Legionella pneumophila is an opportunistic pathogen that causes the potentially fatal pneumonia known as Legionnaires’ disease. The pathology associated with infection depends on bacterial delivery of effector proteins into the host via the membrane spanning Dot/Icm type IV secretion system (T4SS). The Dot/Icm complex of L. pneumophila is one of the largest known T4SSs. The Dot/Icm T4SS has as many as 300 protein substrates, a striking contrast to the H. pylori Cag and B. pertussis Ptl T4SSs, each of which transports only one virulence factor.

Using 3D variability analysis, we reconstructed a total of five maps that displayed differences in the way the outer membrane cap (OMC) and periplasmic ring (PR) were positioned. These maps led to the identification of an approximate 16-fold symmetry about the center of the dome positioned within the OMC. Within this dome there are 16 α-helices that appear nearly identical at this resolution. Indeed, a model of the C-terminal domain of DotG generated in Swiss Model using VirB10 as a template fits into the resolved dome density (Waterhouse et al., 2018). However, we have unexpectedly uncovered that the Dot/Icm incorporates only 16 copies of DotG into the OMC dome out of the 18 DotG copies in the PR, giving rise to another symmetry mismatch within this system. Based on the structure of DotG modeled within the PR (residues 791–824) and the homology model fit into the dome density (consisting approximately of residues 857–1046), we hypothesize that DotG extends from the PR to the dome, though a physical connection between the two structures is not observed. (A) Two DotC were observed in the maps that were reconstructed during 3D variability analysis, one which contains an N-terminal extension (DotCLong) and one which does not (DotCshort). In contrast, the N-terminal extension of DotC was modeled as two relatively large helices positioned near DotG and bridging adjacent asymmetric units. Notably, this portion of DotC was only observed in either four or five of the 13 copies of DotC observed in each map. The movie shows that the OMC dome, OMC disk, and PR of Dot/Icm T4SS can accommodate various orientations in relation to each other that suggest that the complex could undergo a ratcheting motion, in which the dome and PR rotate back and forth about the central axis with the different regions of the complex tethered together by the physical connections across the symmetry mismatches.

>[13x]MRKFILSLSILLSALLVACSSRNHYGDTGSLAGLQAMADSKYTRAQKKQKMGKIREMALKETALSVGAQAGLAWRAKIIDEQLNKQARNLDAIYDFNSLVLEHNILPPVLLEGRNTLNLADAQSIRISDRTYKVAKQAHFITTPPTWRQYLWMDYVKPEAPNVTLLPKTKAEKEIWCIYTERGWKNGIDQANTILEENIARIKEDFGGMILYRKLLAMNMVSPPYVSHTDLGVTGDGSEIHIDDRVLRITALPELNVNSAEWRAAVAKDENALERFKNMEKLANQAKIVITNKSWQPIIAPVS;>MNNNKIVIMFIFSALLAGCAGTMKFKKPPINNPSDDATIKLAEAAVSVSDSMLEMAKVEKVITPPSKDNTLTIPNAYNLQARASVDWSGPIEELTARIAKAAHFRFRVLGKSPSVPVLISISTKDESLAEILRDIDYQAGKKASIHVYPNSQVVELRYAKIYS[26x];>MMAEHDQNNDEYKFAELDSYDMDQAGESDLDSEASYQSGKEGLTKKKDIKRNALIAIGAVVFIMVMYKIIGWMFFSDKSSQVTSKPAIPPVTQVATPQPVQTIPTTTPIQQVQPTTIIEDDPDLKKKVSAIEMTQQSLRSEVNALSEQINAVNNNIKNLNAQIVNLNQIIGNMSNQIARQSEVINVLMARTTPKKVVKVSRPIVQARIIYYIQAVIPGRAWLIGSNGSTLTVREGSKIPGYGMVKLIDSLQGRILTSSGQVIKFSQEDS[31x];>MASKKENLKSLFSNTRTRVIIIFTAALLIIAVVIGFFKIRGATTGSIAAAEVSTVPGGIQSIPGVLDPTAQYAKLQEEQNITQAQVAEKTGGSAIPTIIRTQALGEGVGVIGSQSGVGFAALAQEELGGPQRSLWIQELQDGSCSKSVITKVVNQGAQLTDLKAACSCVQLKDSGYGLQELEQVCECKELKSAGYNARQLKEAGYSAGRLRNCGFDACELRNAGFTAQEMKDGGFSDGELKGAGFSDAEIAKASGLPDGITADDVRKAGCGAAALAKLRQAGVSASAIRKISGCTAEQLKAAGYTAKELKDAGFSAADLRRAGFSAAELKDAGFTARDLLNAGFTPADLAKAGFSDAQIKAAQAELPPGITPQDVKNAGCDVEALKKEREAGVSAALIRQYAGCSAQALKAAGFTDADLANAGFTPAQISAATPLSDAEIKAAGCDPDKLKKLFSAGVSAKRIKELNGCSAEALKAAGYDAQSLLAAGFTPQELLAAGFTPKQLEDAGLNPVSIIADGRVADCSVESLKKARAAGVSALTIKQTLGCSAAALKAAGYTAKELKDAGFTAAELKAAGFSAKELKDAGFTAKELRDAGFSAQELKDVGFSAKDLKDAGFSAAELKAAGFTAAQLKAAGFSAKDLKDAGFSAAELKAAGFSAKELKDAGFSASDLKNAGFSAKELKDAGFSASDLKSAGFSASELKNAGYSADELKKAGYTSAELRNAGFSPQESAVAGLQGPDLQQLDSSITGIPSIPGATPRPTTSDAASSAEQLQAILQKQNEQLAEQKYQQEIQQRTSDMLTAATQLVQDWKQVETQVYTEGTEETKTSGGESAVPGTGTGTGSNNQPVDQGAVSAQNQAIIKTGDIMFAVLDTSVNSDEPGPILATIVTGKLKGSKLIGSFNLPSNADKMVITFNTMSIPGAEKTISISAYAIDPNTARTALASRTNHHYLMRYGSLFASSFLQGFGNAFQSANTTITIGGTGGGNNITVANGVGRSTLENAVIGLATVGKAWSQQAQQLFNTPTTVEVYSGTGLGILFTQDVTTI[34x];>MMKKYDQLCKYCLVIGLTFSMSCSIYAADQSDDAQQALQQLRMLQQKLSQNPSPDAQSGAGDGGDNAASDSTQQPNQSGQANAPAANQTATAGGDGQIISQDDAEVIDKKAFKDMTRNLYPLNPEQVVKLKQIYETSEYAKAATPGTPPKPTATSQFVNLSPGSTPPVIRLSQGFVSSLVFLDSTGAPWPIAAYDLGDPSSFNIQWDKTSNTLMIQATKLYNYGNLAVRLRGLNTPVMLTLIPGQKAVDYRVDLRVQGYGPNAKSMPTEEGIPPSANDLLLHVLEGVPPPGSRRLVVSGGDARAWLSNEKMYVRTNLTILSPGWLASMTSADGTHAYEMQKSPVLLVSWHGKVMQLKVEGL[18x];>MRSLRTNYIYVLFKTTGLLFLLLLSACNRSGYIPENEVPKLPCRVDGACDATIIKMMTDLNKKGIKVASVGQNYLISIPASALFADQSPRLNWASYSLLNEIAAFLKQFRKIAITVTSYSSKYVSVKRERALTLARSRVVSEYLWSQGVDSRIIFTQGLGSDKPITSYTLGGDRSPNARVEITFRRAVA[13x];>[13x]MRNLMRCLIMIKSLIKGVDMSRKLAKTRILGYGLMICFLAGCFHPPYNNFQPDRRAVKRVGVDTGIGAVAGAIASGTASGTLIGAAAGGTVGLVASIYRDSKRKIIRDLQKQDIQYVEYGDTRTLIIPTDKYFMFSSPRLNEICYPGLNNVIRLLNFYPQSTIYVAGFTDNVGSRSHKRKLSQAQAETMMTFLWANGIAAKRLKAEGYGDKNAISDNAIIHGSAQNRRIEIQWFTSPAQPPQPQMAYVK;>[13x]MLKRCYLLILLMFVLASCAHHKPQTPPAEVKKQGTSSTRQFRQVSSFNQIVVQGRLNVNLHTGYNKPEVMLRGDPRDLVQVRTIVKQNTLYVSLGQGYPDYGAVTVDIKTKFLNRFRYEGAGVVTGNNLRTSYLDLYLANEGTTRLAGNIGLQKLEAVGNGVTQINGVSSRNLQIVLKGDPKVLISGFVNLRQLDMYGKGTLSLYWIKSDTLTIRAKKAAKIQLAGIVNRLDVELWDFAQFKGKYLRAQRSFVKTHDKSVAEISAVNHQSSLATDASDIYYYNLSKTRADFMAFNGSVLDMREWGQSDLKDFDRYNKQFP;>MLFLKIKTNQRTTMNILKPKAFLLASVFVLSISPAFAADGCCSKMGGINYCDSSAGRLVCNNGFYSTCYCTRHAVMDLQFLMGCCLWHGGVYPQLNSSGLVVCNDGYVSEECSLQKPVEQISVY[13x]>[2x]MGSITENTSWNKEFSAEAVNGVFVLCKSSSKSCATNDLARASKEYLPASTF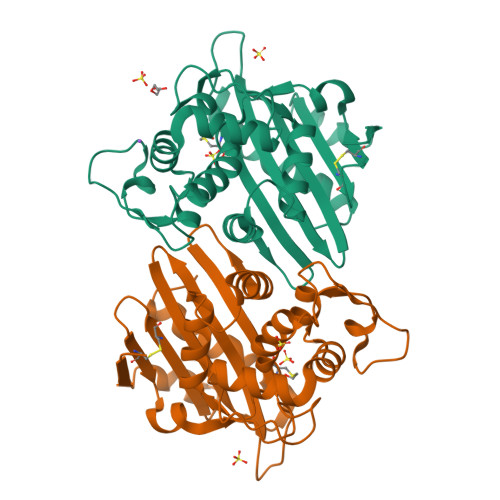KIPNAIIGLETGVIKNEHQVFKWDGKPRAMKQWERDLTLRGAIQVSAVPVFQQIAREVGEVRMQKYLKKFSYGNQNISGGIDKFWLEGQLRISAVNQVEFLESLYLNKLSASKENQLIVKEALVTEAAPEYLVHSKTGFSGVGTESNPGVAWWVGWVEKETEVYFFAFNMDIDNESKLPLRKSIPTKIMESEGIIG>MAHHHHHHMKDHTIPLTLISILADGEFHSGEQLGEQLGMSRAAINKHIQTLRDWGVDVFTVPGKGYSLPEPIHLLDEKKISQEIDHGRVTVLPVIDSTNQYLLDRLDELTSGDACVAEYQQAGRGRRGRKWFSPFGANLYLSMYWRLEQGPAAAIGLSLVIGIVIAEVLQQLGAEQVRVKWPNDIYLQDRKLSGILVELTGKTGDAAQIVSGAGINLVMRRVESDVVNQGWISLQEAGVVIDRNLLAARLIKELRLGLELFEQEGLAPYLPRWEKLDNFIHRPVKLIIGD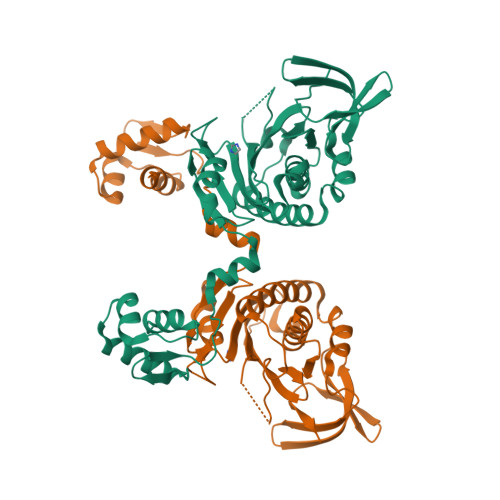KEIYGISRGIDAQGALLLEQDGVIKAWVGGEISLRSAE[2x]>[2x]MSKPQPIAAANWKCNGSQQSLSELIDLFNSTSINHDVQ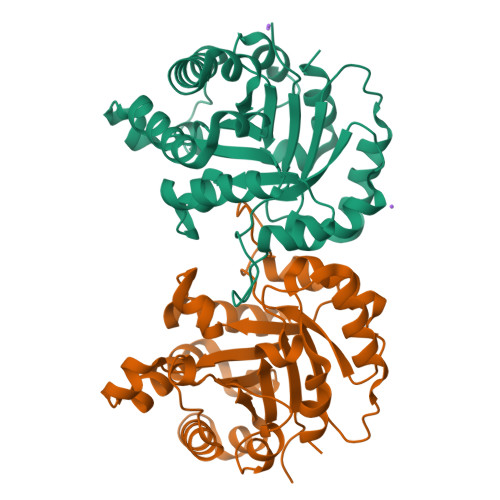CVVASTFVHLAMTKERLSHPKFVIAAQNAIAKSGAFTGEVSLPILKDFGVNWIVLGHSERRAYYGETNEIVADKVAAAVASGFMVIACIGETLQERESGRTAVVVLTQIAAIAKKLKKADWAKVVIAYEPVWAIGTGKVATPQQAQEAHALIRSWVSSKIGADVAGELRILYGGSVNGKNARTLYQQRDVNGFAVGGASLKPEFVDIIKATQ In the RAM network, the hippo-like kinase Kic1 activates the NDR-related kinase Cbk1, which forms a complex with the coactivator protein Mob2. Here we describe the crystal structure of the yeast Cbk1–Mob2 complex, providing what is to our knowledge the first structural template for an NDR/LATS kinase–Mob coactivator complex. In each structure, Mob2 binds to the conserved N-terminal extension of the Cbk1 AGC kinase domain, a region previously identified as the site by which NDR kinases bind Mob proteins. In all three structures, the Cbk1 HM peptide is wedged into a binding slot in the deep cleft formed by the kinase’s αMob helix, N-linker region, and N-terminal catalytic domain lobe.

In addition to Cbk1 intact in its HM region, we used a variant in which threonine 743 was replaced by glutamic acid, an activating substitution that is at least partially phosphomimetic. We also solved the structure of Cbk1(HM-E)–Mob2 in a crystal form that diffracted to 3.6 Å, containing two Cbk1(HM-E)–Mob2 complexes in the asymmetric unit related by noncrystallographic symmetry (NCS). Cbk1’s activation loop forms multiple different structures: the higher resolution Cbk1(HM-E)–Mob2 crystallographic model captures two of these conformations displayed by the two NCS-related models. In one form, structured parts of the activation loop occupy the substrate-binding pocket and thus occlude access to the catalytic site, similar to the structure of PKA complexed with an alpha helical peptide inhibitor. In the other complex, the activation loop is not present in the substrate-binding region. We suggest that this is an auto-inhibited form of the kinase, while the other state seen in one of the two complexes present in Cbk1(HM-E) crystals may be competent to bind substrates containing basic amino acids (right). Although crystal packing interactions around the kinase activation loop are clearly different for the two complexes of the Cbk1(HM-E)–Mob2 model, it is likely that the extended activation loop of NDR/LATS kinases switches them between an inhibited and open state, with phosphorylation of the conserved autoregulatory site S570 (near AMPPNP in Fig 2C, left) alleviating the pseudo-substrate-based inhibition exerted by the inhibitory helix (αINH). In our crystal structures, unphosphorylated wild-type (WT) HM region (HM-T) and HM region with glutamic acid substitution (HM-E) associate with the Mob2-supported binding site in a similar manner. Similar MD analysis of the Cbk1(HM-E)–Mob2 structure indicates that HM-E also has more restrained movement of the HM region within the binding slot than HM-T, but slot compression was significantly less pronounced compared to HM-P. This suggests that HM-E is only a partial substitute for HM-P.

>GSSPVQSGFNNGTISNYMYFERRPDLLTKGTQDKAAAVKLKIENFYQSSVKYAIERNERRVELETELTSHNWSEERKSRQLSSLGKKESQFLRLRRTRLSLEDFHTVKVIGKGAFGEVRLVQKKDTGKIYAMKTLLKSEMYKKDQLAHVKAERDVLAGSDSPWVVSLYYSFQDAQYLYLIMEFLPGGDLMTMLIRWQLFTEDVTRFYMAECILAIETIHKLGFIHRAIKPDNILIDIRGHIKLSDFGLSTGFHKTHDSNYYKKLLQQDEATNGISKPGTYNANTTDTANKRQTMVVDSISLTMSNRQQIQTWRKSRRLMAYSTVGTPDYIAPEIFLYQGYGQECDWWSLGAIMYECLIGWPPFCSETPQETYRKIMNFEQTLQFPDDIHISYEAEDLIRRLLTHADQRLGRHGGADEIKSHPFFRGVDWNTIRQVEAPYIPKLSSITDTRFFPTDELENVPDSPAMAQAAKQREQMTKQGGSAPVKEDLPFIGYEYSRFDYLTRKNAL[2x];>GSRNKHHSPKRHSQTSFPAQKSTPQSQQLTSTTPQSQQQEASERSESQQIMFLSEPFVRTALVKGSFKTIVQLPKYVDLGEWIALNVFEFFTNLNQFYGVVAEYVTPDAYPTMNAGPHTDYLWLDANNRQVSLPASQYIDLALTWINNKVNDKNLFPTKNGLPFPQQFSRDVQRIMVQMFRIFAHIYHHHFDKIVHLSLEAHWNSFFSHFISFAKEFKIIDRKEMAPLLPLIESFEKQGKIIYN[2x]>[2x]MEAVVISGRKLAQQIKQEVRQEVEEWVASGNKRPHLSVILVGENPASHSYVLNKTRAAAVVGINSETIMKPASISEEELLNLINKLNNDDNVDGLLVQLPLPEHIDERRICNAVSPDKDVDGFHVINVGRMCLDQYSMLPATPWGVWEIIKRTGIPTLGKNVVVAGRSKNVGMPIAMLLHTDGAHERPGGDATVTISHRYTPKEQLKKHTILADIVISAAGIPNLITADMIKEGAAVIDVGINRVHDPVTAKPKLVGDVDFEGVRQKAGYITPVPGGVGPMTVAMLMKNTIIAAKKVLRLEEREVLKSKELGVATN

The folate metabolism enzyme MTHFD2 (methylenetetrahydrofolate dehydrogenase/cyclohydrolase) is consistently overexpressed in cancer but its roles are not fully characterized, and current candidate inhibitors have limited potency for clinical development. Indeed, the one-carbon metabolism enzyme MTHFD2 stands out as the most consistently overexpressed metabolic enzyme across human tumors. MTHFD2 enzymatic function supports rapid cell proliferation during early embryogenesis, after which it is replaced by the mitochondrial protein MTHFD2L in healthy mature tissue.

The tool compound TH7299, as well as two of the most promising candidates, TH9028 and TH9619, were chosen to investigate the MTHFD2 mechanism of action and cancer biology. Furthermore, we determined the cocrystal structures of TH7299, TH9028 and TH9619 in complexes with human MTHFD2 to assess their binding mode and identify critical interactions in the binding pocket. At a predetermined temperature of 57 °C, isothermal dose–response fingerprint (CETSAITDRF) analysis of TH7299, TH9028 and TH9619 in HL-60 cells accurately reflected their relative potencies in biochemical and viability assays, as well as demonstrating the difference in target stabilization potential for TH9619 in nontumorigenic lymphoblastoid cell line (LCL)-889 cells compared with HL-60 AML cells. In contrast, TH9028 and TH9619 showed overall strong antiproliferative efficacy in AML cells and T-ALL Jurkat cells comparable to standard-of-care compounds, with reduced effect on LCL viability. Treatment with TH7299 resulted in approximately 50% reduction of RF speed and significantly shorter DNA fibers; meanwhile supplementation with thymidine was sufficient to fully rescue replication speeds. Similar fork speed reductions were also observed on TH9028 treatment in HL-60 and THP-1 cells. Although MTX and VE-821 significantly blocked DNA RF progression in both cancer and nontumorigenic cells, MTHFD2 inhibitors effectively impaired DNA replication only in AML cells, sparing nontumorigenic lymphocytes. The same cancer selectivity was observed for TH9028.(1~{S},2~{R},4~{R})-1-methyl-2-[(2-methylphenyl)methoxy]-4-propan-2-yl-7-oxabicyclo[2.2.1]heptane | 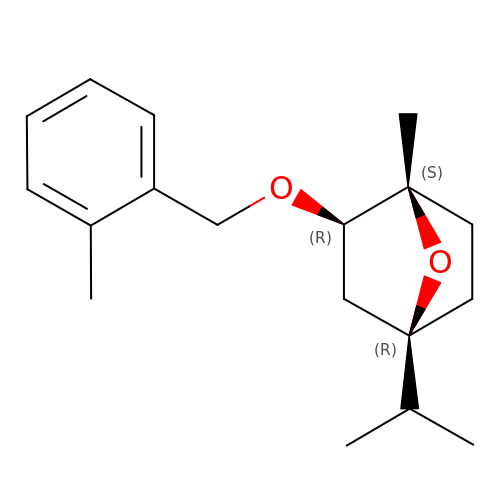C18 H26 O2 | QMTNOLKHSWIQBE-UQJFVLDMSA-N> MNSPISPIETVPVKLKPGMDGPKVKQWPLTEEKIKALVEICTEM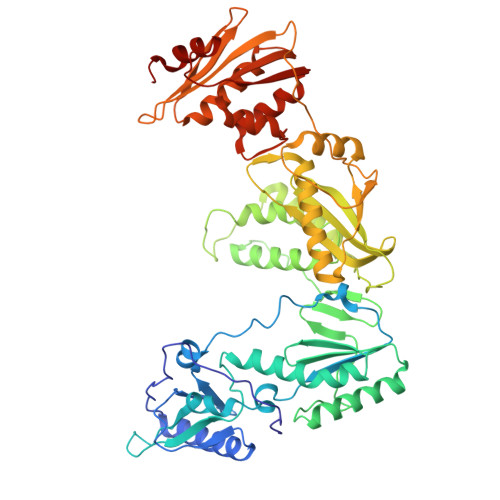EKEGKISKIGPENPYNTPVFAIKKKDSTKWRKLVDFRELNKRTQDFWEVQLGIPHPAGLKKKKSVTVLDVGDAYFSVPLDEDFRKYTAFTIPSINNETPGIRYQYNVLPQGWKGSPAIFQSSMTKILEPFRKQNPDIVIYQYMDDLYVGSDLEIGQHRTKIEELRQHLLRWGLTTPDKKHQKEPPFLWMGYELHPDKWTVQPIVLPEKDSWTVNDIQKLVGKLNWASQIYPGIKVRQLCKLLRGTKALTEVIPLTEEAELELAENREILKEPVHGVYYDPSKDLIAEIQKQGQGQWTYQIYQEPFKNLKTGKYARMRGAHTNDVKQLTEAVQKITTESIVIWGKTPKFKLPIQKETWETWWTEYWQATWIPEWEFVNTPPLVKLWYQLEKEPIVGAETFYVDGAANRETKLGKAGYVTNRGRQKVVTLTDTTNQKTELQAIYLALQDSGLEVNIVTDSQYALGIIQAQPDQSESELVNQIIEQLIKKEKVYLAWVPAHKGIGGNEQVDKLVSAGIRKVL> MKVLGVVVEYNPFHNGHLYHLTSARELVKPDYTIAVMSGNFCQRGEPAVIDKFARAEIALRMGVDVVLELP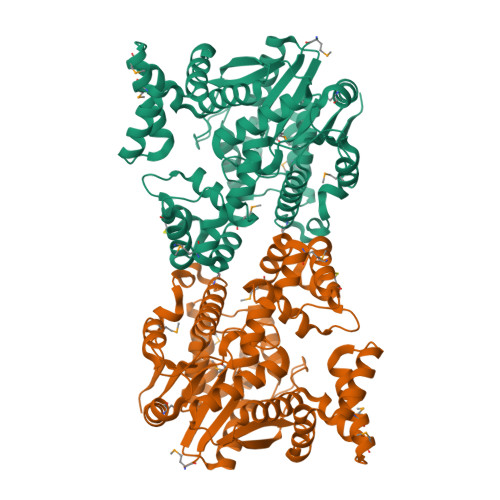VVFATQDAGGFAFGAVCVLDATGVVTDVVFGSESNDIEFLQRVARILYEQPDEYQKFLHEELKKGYSFPNARKYALMRYFSMKGWNEEEVLKLEKSNDILGVEYIHSALKIGSNIRFHTIKRVGAEEKDTSFRGRFSSATAIRNLMREKRWEEVRDSLPEDSFEILMREINEGRGPVFLENMGDFLLSFFRLKNMDFFEKIHGFSEGLEKRFHVCARQTGSYRDFLECVKAKRFTFSRIRRLALFSVFEVNKEFVEKSNTKGPQYIRILGFTEKGREILSLMRKKAKLPIVTNMSLYRKVLEKTDLPVDKQLFLEQIDLDVKATNFYSMFFPSVEQRCGERDFSIHPIFLRTEM>RGLASKKTTTVGVIIPDISNIFYAELARGIEDIATMYKYNIILSNSDQNQDKELHLLNNMLGKQ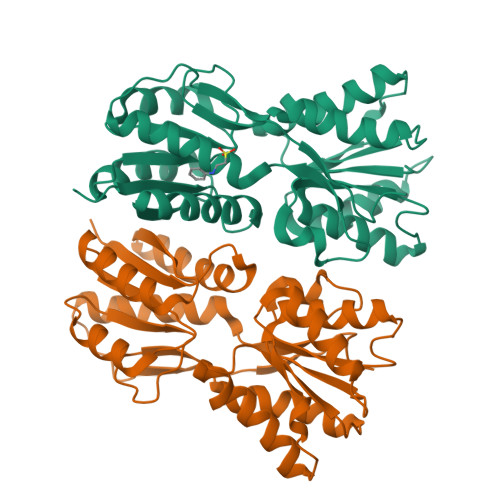VDGIIFMSGNVTEEHVEELKKSPVPVVLAASIESTNQIPSVTIDYEQAAFDAVQSLIDSGHKNIAFVSGTLEEPINHAKKVKGYKRALTESGLPVRDSYIVEGDYTYDSGIEAVEKLLEEDEKPTAIFVGTDEMALGVIHGAQDRGLNVPNDLEIIGFDNTRLSTMVRPQLTSVVQPMYDIGAVAMRLLTKYMNKETVDSSIVQLPHRIEFRQSTK[6x]> TAHSNSQALLDL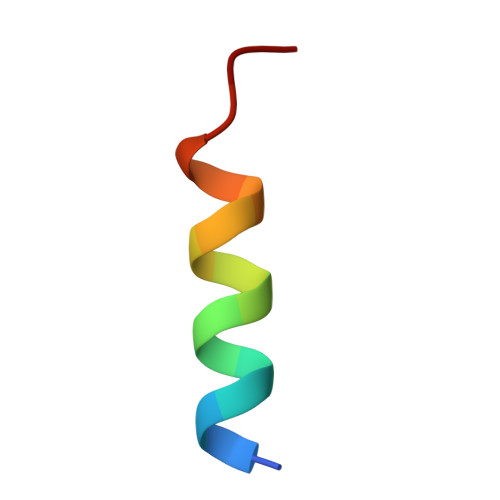LKKPT DNA synthesis during replication relies on RNA primers synthesised by the primase, a specialised DNA-dependent RNA polymerase that can initiate nucleic acid synthesis de novo. In archaeal and eukaryotic organisms, the primase is a heterodimeric enzyme resulting from the constitutive association of a small (PriS) and large (PriL) subunit. The ability of the primase to initiate synthesis of an RNA primer depends on a conserved Fe-S domain at the C-terminus of PriL (PriL-CTD). Recently, it has been reported that a conserved sequence in the C-terminal region of archaeal and eukaryotic PriL folds in a separate domain around an Fe-S cluster cofactor coordinated by four conserved cysteines (PriL-Carboxy-Terminal Domain; PriL-CTD).

The most conspicuous feature of the PriL-CTD architecture is its organisation in two largely independent domains, arranged as triangular wedges joined via their thin ends. The larger N-terminal domain spans residues 321 to 433 whereas the smaller C-terminal domain includes residues 434 to 512. When the structure of the yeast PriL-CTD was compared to protein structures in Protein Data Bank in Dali no significant structural similarity with known Fe-S proteins was detected, confirming that the PriL-CTD represents a novel type of Fe-S cluster-binding domain. Surprisingly, the search identified significant matches, with Z-scores ranging from 8.0 to 6.1, between the larger N-terminal domain of PriL-CTD and members of the DNA photolyase/cryptochrome family, DNA repair enzymes that revert the accidental cross-linking of adjacent bases, such as cyclobutane-pyrimidine dimers (CPD) and pyrimidine-pyrimidone (6-4) dimers, caused by ultraviolet light. The portion of the DNA photolyase/cryptochrome structure identified as similar to the N-terminal domain of PriL-CTD encompasses its active site and includes the FAD- and DNA-binding sites. The mode of binding of single-stranded (ss) DNA and FAD observed in the co-crystal structure of the DASH cryptochrome 3 from A. thaliana suggests that the PriL-CTD could adopt a similar mode of interaction with the template DNA and ribonucleotides during de novo RNA synthesis. In particular, the spacial relationship between FAD and the extruded, cross-linked pyrimidine dimer observed in the active site of DNA photolyase suggests a possible arrangement for the pairing of the first dinucleotide of the RNA primer onto template DNA during the initiation step catalysed by the primase. The structural similarity of the N-terminal domain of PriL-CTD with the active site of DNA photolyase and the analysis of its electrostatic potential and surface-residue conservation predicts that the PriL-CTD should possess a DNA binding ability. The rather low DNA-binding affinity of the PriL-CTD agrees with previous biochemical evidence that the DNA-binding ability of the eukaryotic primase is mainly provided by the small subunit PriS.

>SDEINAQSVWSEEISSNYPLCIKNLMEGLKKNHHLRYYGRQQLSLFLKGIGLSADEALKFWSEAFTNMTMEKFNKEYRYSFRHNYGLEGNRINYKPWDCHTILSKPRPGRGDYHGCPFRDWSHERLSAELRSMKLTQAQIISVLDSCQKGEYTIACTKVFEMTHNSASADLEIGEQTHIAHPNLYFERSRQLQK[2x]>MHHHHHHHKPEDFRASTQRPFTGEEYLKSLQDGREIYIYGERVKDVTTHPAFRNAAASVAQLYDALHKPEMQDSLCWNTDTGSGGYTHKFFRVAKSADDLRQQRDAIAEWSRLSYGWMGRTPDYKAAFGCALGANPGFYGQFEQNARNWYTRIQETGLYFNHAIVNPPIDRHLPTDKVKDVYIKLEKETDAGIIVSGAKVVATNSALTHYNMIGSGSDLGSGSDPDFALMFVAPMDADGVKLISR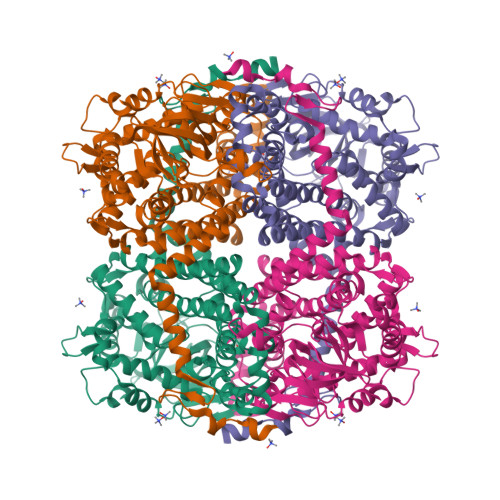ASYEMVAGATGSPYDYPLSSRFDENDAILVMDNVLIPWENVLIYRDFDRCRRWTMEGGFARMYPLQACVRLAVKLDFITALLKKSLECTGTLEFRGVQADLGEVVAWRNTFWALSDSMCSEATPWVNGAYLPDHAALQTYRVLAPMAYAKIKNIIERNVTSGLIYLPSSARDLNNPQIDQYLAKYVRGSNGMDHVQRIKILKLMWDAIGSEFGGRHELYEINYSGSQDEIRLQCLRQAQNSGNMDKMMAMVDRCLSEYDQDGWTVPHLHNNDDINMLDKLLK[2x]>UUGCGUCGUUCCGGAAA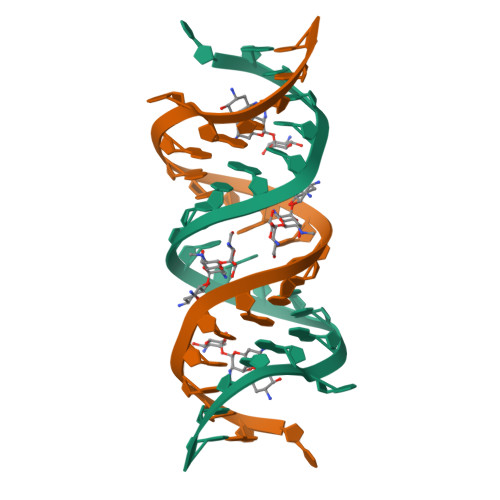AGUCGC[2x]> MAHHHHHHDDDDKIRTLPGEGTQVHPRAPLLQILKVAGAQEEVFTLKEVMHYLGQYIM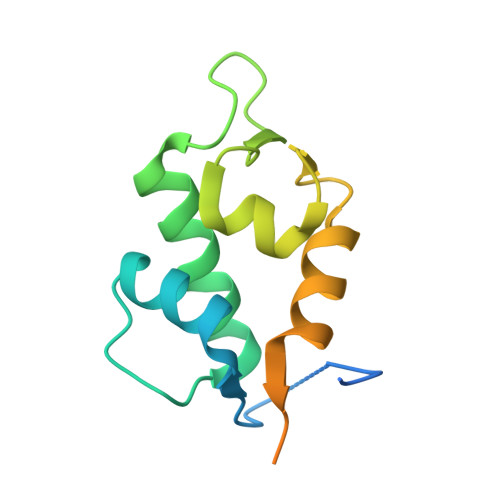MKQLYDKQRQHIVHCHDDPLGELLEVGSFSVKNPSPVYEMLKRNLVILNNSDAAKNLSVGKDSNESPSEDPGQVSSGSINSA> MLPEKSEIVVIGGGIVGVTIAHELAKRGEEVTVIEKRFIGSGSTFRCGTGIRQQFNDEANVRVMKRSVELWKKYSEEYGFSFKQTGYLFLLYDDEEVKTFKRNIEIQNKFGVPTKLITPEEAKEIVPLLDISEVIAASWNPTDGKADPFEATTAFAVKAKEYGAKLLEYTEVKGFLIENNEIKGVKTNKGIIKTGIVVNATNAWANLINAMAGIKTKIPIEPYKHQAVITQPIKRGTINPMVISFKYGHAYLTQTFHGGIIGGIGYEIGPTYDLTPTYEFLREVSYYFTKIIPALKNLLILRTW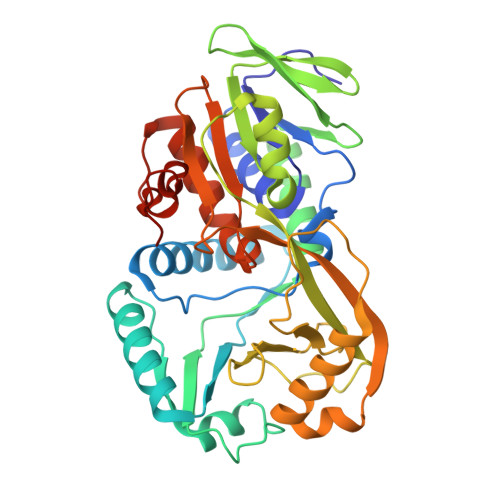AGYYAKTPDSNPAIGRIEELNDYYIAAGFSGHGFMMAPAVGEMVAELITKGKTKLPVEWYDPYRFERGELRTAALQMG Previously, we described the isolation of one such crystal protein, designated Cry51Aa2, with activity towards the hemipteran pests L. hesperus and L. lineolaris. The structure reveals an elongated predominantly β-stranded structure with similarities to other bacterial β pore-forming proteins. The structure of Cry51Aa2 closely resembles that of Cry51Aa1, which is expected as these two proteins have high sequence homology (97.7% identity).

Crystal 1 was used to solve the structure by SeMet multi-wavelength anomalous dispersion (MAD) phasing methods. Cry51Aa2 protein crystallizes in tetragonal crystal lattices (a,b=55–56 Å, c=209–210 Å, all angles 90°) and in the P43212 space group. Recently, the structure of the closely related Cry51Aa1 (1.65 Å) protein was published. A super-positioning alignment of Cry51Aa1 onto the SeMet-Cry51Aa2-L11M structure coordinates conducted using the align program in PyMOL revealed that the structures have a pair-wise root mean square difference in α-carbon positions of 0.57 Å (using 291 α-carbon pairs). Also, Cry51Aa1 and Cry51Aa2 proteins crystallize in nearly identical tetragonal crystal lattices and in the identical space group. Substitutions at positions 93, 95, 147, 149 and 251 reside on adjacent antiparallel β-strands in the region adjacent to the putative amphipathic pore-forming loop (residues 112–140) and define a second region within the Cry51Aa2 structure impacting insecticidal activity. Surface-exposed side-chain substitutions in residues engaged in antiparallel β-sheets, as is the case here, should not impact the lateral hydrogen bonds which stabilize the β-sheet, but could impact other processes such as protein oligomerization or pore formation. Finally, the R273W substitution resulting in increased Lygus activity (for example, Cry51Aa2.834_15 in Table 1) is located in the tail region of the molecule and may promote interactions with the target cell membrane due to increased hydrophobicity at that position.

> MAILDLKSLVMNAINYWGPKNNNGIQGGDFGYPISEKQIDTSIITFTHPRLIPYDLTIPQNLETIFTTTQVLTNNTDLQQSQTVSFAKKTTTTTSTSTTNGWTEGGKISDTLEEKVSVSIPFIGEGGGKNSTTIEANFAHNSSTTTFQQASTDIEWNISQPVLVPPSKQVVATLVIMGGNFTIPMDLMTTIDSTEHYSHYSGYPILTWISSPDNSYSGPFMSWYFANWPNLPSGFGPLNSDNTVTYTGSVVSQVSAGVYATVRFDQYDIHNLRTIEKTWYARHATLHNGKKISINNVTEMAPTSPIKTN>MASMTGGQQMGRGSMSTKAIYPGTFDPITNGHIDIITRAASMFDRVILAIAASPSKKPMFDLEERVALATTALQHLPNVEVMGFSDLMA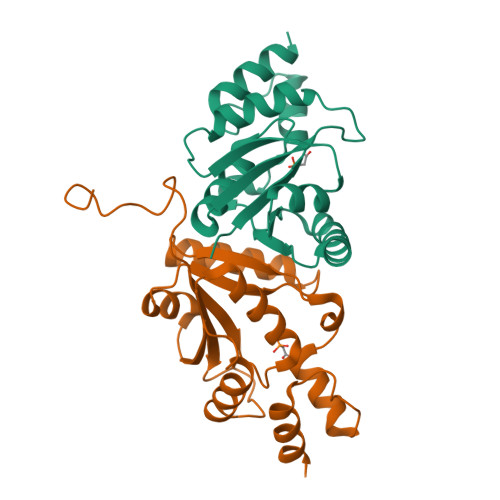NFARAQQANILIRGLRAVADFEYEMQLAHMNRHLMPELESVFLMPSKEWSFISSSLVKEVARHAGDVTHFLPANVHQALMEKLK[6x]>[6x]MEKQSSLETQAFSFAEEFAWDYFSRYP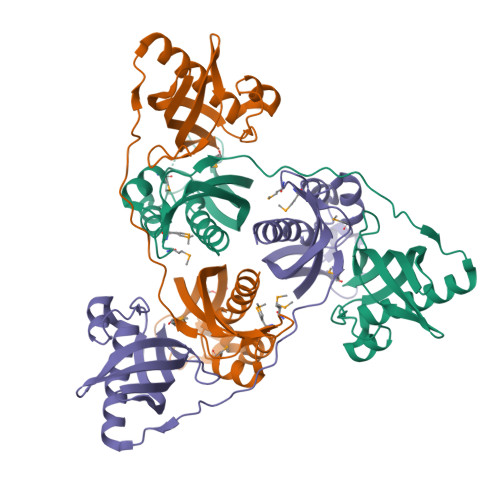SDTQDFVRRITKYTTEQLANEMNNGTYSDVIYTSAFYFEKYSENQVNVSVKARVRVYTPKAGQEQTPQDQLQYDTNLVDYYLEVPIVFDKDMNMAVDALPVMTAPPEKAYFKNKEFSGTSENDADKTKKITDSVSQFFKAYYEQNQTQIDYFLVDGADIKGAGQKFSFNKIDRINIYKLSDKEFLAIVDLNVDSFGNAIKQGFNLTVVQEGDKFLVKTLEPRTSNIDLNNKSNN>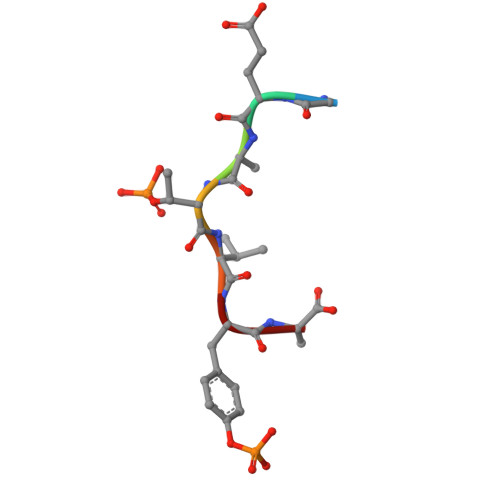 GEATVYA>VNFPNIPAEGAQFRLRARDTGYVIYSRTENPPLVWQYNGPPYDDQLFTLIYGTGPHQNLYAIKSVPNGRVLFSRTSASPHVGNIAGDGTYNDNWFQFIQDDNDPNSFRIYSLA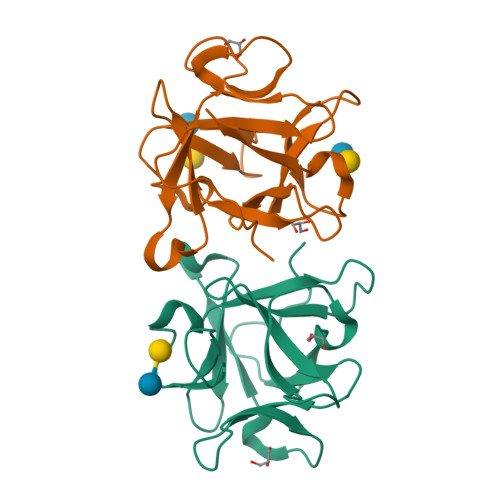SDTVLYSRTTPDPQFGNYTGAKYDDQLWHFELV[4x]>[2x]MAITAKPKAGVWAVLWDLLTTVDHKKIGLMYTATAFFAFALAGVFSLLIRTQLAVPNNQFLTGEQYNQILTLHGATMLFFFIIQAGLTGFGNFVVPLMLGARDVALPRVNAFSYWAFLGAIVLALMSYFFPGGAPSVGWTFYYPFSAQSESGVDFYLAAILLLGFSSLLGNANFVATIYNLRAQGMSLWKMPIYVWSVFAASVLNLFSLAGLTAATLLVLLERKIGLSWFNPAVGGDPVLFQQFFWFYSHPTVYVMLLPYLGILAEVASTFARKPLFGYRQMVWAQMGIVVLGTMVWAHHMFTVGESTLFQIAFAFFTALIAVPTGVKLFNIIGTLWGGKLQMKTPLYWVLGFIFNFLLGGITGVMLSMTPLDYQFHDSYFVVAHFHNVLMAGSGFGAFAGLYYWWPKMTGRMYDERLGRLHFWLFLVGYLLTFLPQYALGYLGMPRRYYTYNADIAGWPELNLLSTIGAYILGLGGLVWIYTMWKSLRSGPKAPDNPWGGYTLEWLTASPPKAHNFDVKLPTEFPSERPLYDWKKKGVELKPEDPAHIHLPNSSFWPFYSAATLFAFFVAVAALPVPNVWMWVFLALFAYGLVRWALEDEYSHPVEHHTVTGKSNA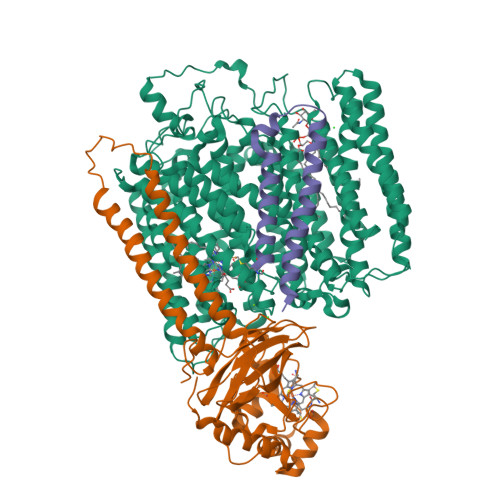WMGMAWFIVSEVGLFAILIAGYLYLRLSGAATPPEERPALWLALLNTFLLVSSSFTVHFAHHDLRRGRFNPFRFGLLVTIILGVLFFLVQSWEFYQFYHHSSWQENLWTAAFFTIVGLHGLHVVIGGFGLILAYLQALRGKITLHNHGTLEAASMYWHLVDAVWLVIVTIFYVW;>[2x]MQRSFAALGLWGLSLAQEAHRVAITHPGGSFNQEVAFLFPWVYFFSFLIFLVVAGSLAYVTWKFRARPEDQEEPPQIHGNDRLEVVWTLIPLAIVFVLFGLTAKALIQVNRPIPGAMKVEVTGYQFWWDFHYPELGLRNSNELVLPAGVPVELEITSKDVIHSFWVPGLAGKRDAIPGQTTRISFEPKEPGLYYGFCAELCGASHARMLFRVVVLPKEEFDRFVEAAKASPAPVADERGQQVFQQNCAACHGVARSMPPAVIGPELGLWGNRTSLGAGIVENTPENLKAWIRDPAGMKPGVKMPGFPQLSEEDLDALVRYLEGLKVEGFDFGALPKF;>MVYIALFALGAALVTLFFYLILNPRVLTTEGETFDLRFVLFMLLLILLAAGTVALMLLIGKAHHLL[2x]> MYVPARSLARKSVVLTDGTVVGTLYNITVDFKTGTIVNLLVKPENEIPDFKKEEGLYIIPFECVRSLK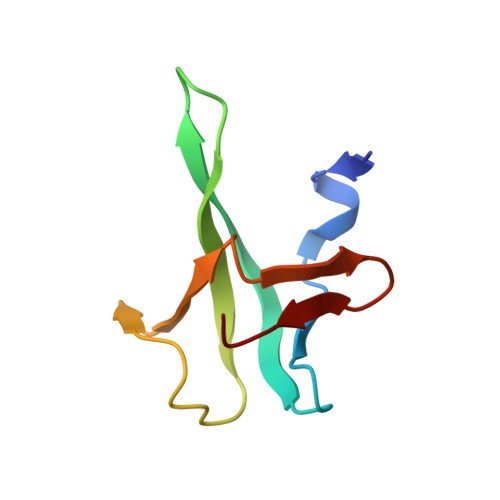DFIVVDRR> HHHHHHGSANKAVNDFILAMNYDKKKLLTHQGESIENRFIKEGNQLPDEFVVIERKKRSLSTSTSDISVTATNDSRLYPGALLVVDETLLENNPTLLAVDRAPMTYSIDLPGLASSDSFLQVEDPSNSSVRGAVNDLLAKWHQDYGQVNNVPARMQYEKITAHSMEQLKVKFGSDFEKTGNSLDIDFNSVHSGEKQIQIVNFKQIYYTVSVDAVRNPGDVFQDTVTVEDLKQRGISAERPLVYISSVAYGRQVYLKLETTSKSDEVEAAFEALIKGVKVAPQTEWKQILDNTEVKAVILGGDPSSGARVVTGKVDMVDDLIQEGSRFTADHPGLPISYTTSFLRDNVVATFQNSTDYVETKVTAYRNGDLLLDHSGAYVAQYYITWD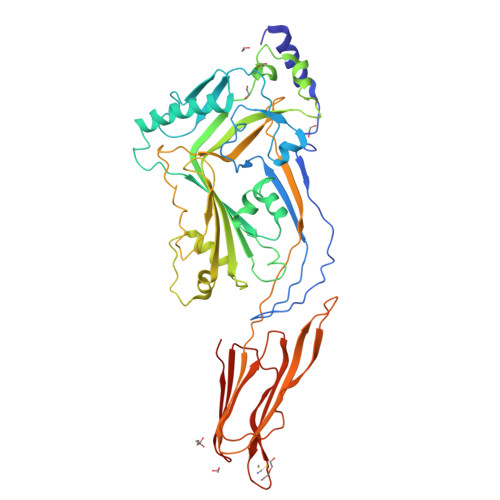ELSYDHQGKEVLTPKAWDRNGQDLTAHFTTSIPLKGNVRNLSVKIRECTGLAWEWWRTVYEKTDLPLVRKRTISIWGTTLYPQVEDKVEN>MTTGLSTAGAQDIGRSSVRPYLEECTRRFQEMFDRHVVTRPTKVELTDAELREVIDDCNAAVAPLGKTVSDERWISYVGVVLWSQSPRHIKDMEAFKAVCVLNCVTAVWDDMDPALHDFGLFLPQLRKICEKYYGPEDAEVAYEAARAFVTSDHMFRDSPIKAALCTTSPEQYFRFRVTDIGVDFWMKMSYPIYRHPEFTEHAKTSLAARMTTRGLTIVNDFYSYDREVSLGQITNCFRLCDVSDETAFKEFFQARLDDMIEDIECIKAFDQLTQDVFLDLIYGNFVWTTSNKRYKTAVNDVNSRIQAAALEHHHHHH[2x]

To elucidate the dynamic interactions of TPSs with their substrates during catalysis, we investigated the bacterial diterpene synthase CotB2 as a model system. CotB2 adopts an α-helical bundle fold that is conserved among class I TPSs (PDB-ID 4OMG17). The CotB2 protein sequence exhibits a modified aspartate-rich DDXD motif12 deviating from the conventional DDXXD motif and the NSE triad NDXXSXX(R,K)(E,D) as found in bacteria and fungi, that is altered to a DTE triad in plants. Upon substrate and Mg2+ binding, TPSs undergo a discrete conformational change from an open, catalytically inactive one to a catalytically active closed conformation.

To comprehend the state of the CotB2wt•Mg2+B•GGSDP structure, we determined the structure of CotB2F107A under a Mg2+-rich condition (CotB2F107A•Mg2+B). Interestingly, a single magnesium-ion (Mg2+B) was bound to the active site, coordinated by the residues N220, S224 and E228 of the NSE motif and two water molecules. Therefore, we suggest the binding of Mg2+B to be the first step in preparing CotB2 for substrate binding. The position of the Mg2+B matches perfectly with that in the CotB2wt•Mg2+B•GGSDP structure. Moreover, the conformation of the Mg2+B coordinating amino acids are oriented in the same manner as there are two water molecules in our structure that mimic the oxygens of the diphosphate group in CotB2wt•Mg2+B•GGSDP. In the structure of CotB2F107A•Mg2+B the salt-bridge of D111 and R294 has not yet been established and the remaining C-terminus could not be resolved. This suggests, that the accurate positioning of the diphosphate moiety is required for the formation of the latter salt-bridge. The overall structure of CotB2wt•Mg2+B•GGSDP is most similar to CotB2wt and CotB2F107A•Mg2+B as indicated by a low root-mean-square deviation. Hence, the structures are likely different pre-catalytic states of CotB2. The CotB2 mutation F107A afforded cembrene A as a product.> MMEEQELTSACKKSLVRIFKICDIDGDNLLNDYELNLFQRRCFNTPLQPQILDEVKAVIQKNVPDGIYNDAVTLKGFLFL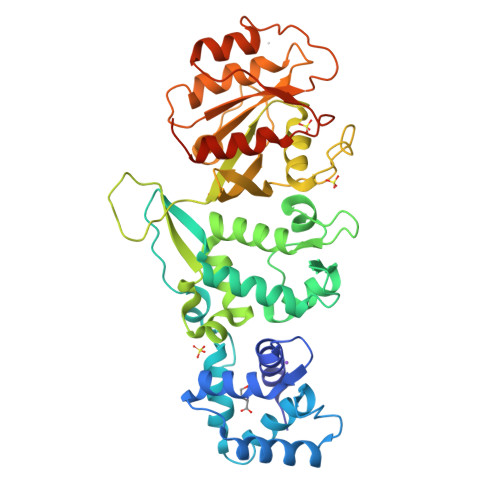HCLFIQRGRNETTWAVLRRFGYNDQLEMCQEYLRPPLKIPPGSSTELSHRGQQFLIAVFERYDRDGDGALSPEEHKMLFSTCPAAPWSYSTDIRKSCPINETTGWVTLHGWLCRWTLMTLIDVVKTMEYLAYLGFNVHENDSQLAAIHVTRERRIDLAKRQSSRSVYKCHVIGPKGSGKTGMCRGFLVEDMHKLIGKEFKTNVVNCINSVQVYGQEKHLILRDIDVRHALDPLQPQEVNCDVACLVYDSSNPRSFEYVARIYIKYYAESKIPVMIVGTKCDMDERRQDYLMQPSEFCDKYKLLPPHLFSLKTNKKELYTKLATMAAFPHLRQFGLMTHHHHHH> VVGGTEAQRNSWPSQISLQYRSGSSWAHTCGGTLIRQNWVMTAAHCVDRELTFRVVVGEHNLNQNDGTEQYVGVQKIVVHPYWNTDDVAAGYDIALLRLAQSVTLNSYVQLGVLPRAGTILA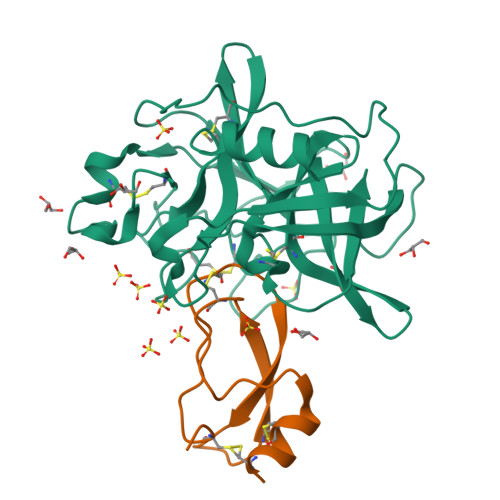NNSPCYITGWGLTRTNGQLAQTLQQAYLPTVDYAICSSSSYWGSTVKNSMVCAGGDGVRSGCQGDSGGPLHCLVNGQYAVHGVTSFVSRLGCNVTRKPTVFTRVSAYISWINNVIASN;> SICSEPKKVGRCLGYFPRFYFDSETGKCTPFIYGGCGGNGNNFETLHQCRAICRA>[2x]MSKQFVRSAKNMMKGYSSTQVLVRDATANDSRTPSIDTLDDLAQRSYDSVDFFEIMDMLDKRLNDK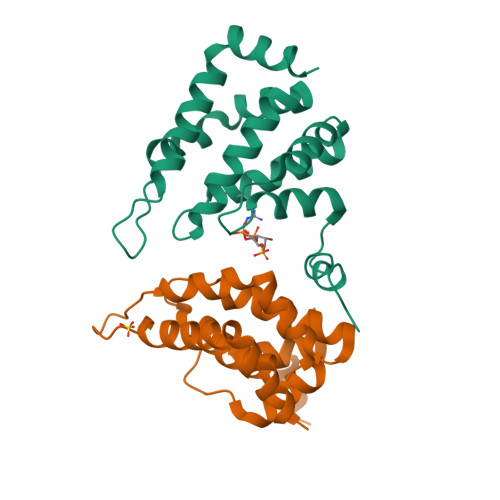GKYWRHVAKSLTVLDYLVRFGSENCVLWCRENFYVIKTLREFRHENESGFDEGQIIRVKAKELVSLLNDEERLREERSMNTRNRRANRAA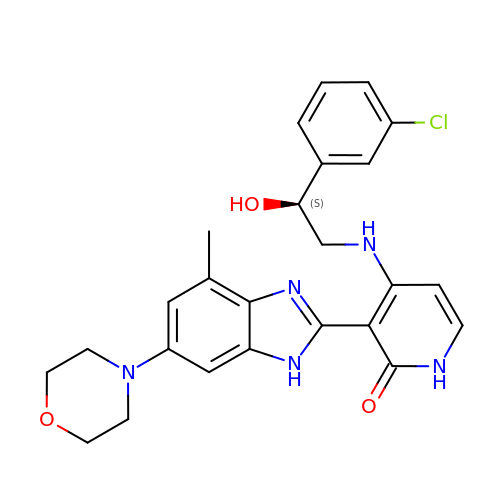(3M)-4-{[(2S)-2-(3-chlorophenyl)-2-hydroxyethyl]amino}-3-[4-methyl-6-(morpholin-4-yl)-1H-benzimidazol-2-yl]pyridin-2(1H)-one | C25 H26 Cl N5 O3 | ZWVZORIKUNOTCS-OAQYLSRUSA-N>GSHMGGVEVLEVKTGVDAITEVECFLNPEMGDPDENLRGFSLKLSAENDFSSDSPERKMLPCYSTARIPLPNLNEDLTCGNLLMWEAVTVQTEVIGITSMLNLHAGSQKVHEHGGGKPIQGSNFHFFAVGGDPLEMQGVLMNYRTKYPDGTITPKNPTAQSQVMNTDHKAYLDKNNAYPVECWVPDPSRNENTRYFGTFTGGENVPPVLHVTNTATTVLLDEQGVGPLCKADSLYVSAADICGLFTNSSGTQQWRGLARYFKIRLRKRSVKNPYP[5x]

The human polyomavirus BK Virus (BKPyV) is a non-enveloped, double-stranded DNA (dsDNA) virus that belongs to the family Polyomaviridae. A polyomavirus capsid consists of 72 pentamers of the major capsid protein VP1. Gangliosides were found to mediate cell attachment of BKPyV, and gangliosides GD1b and GT1b were later shown to function as specific receptors for BKPyV. Crystal structures of Polyoma, SV40, MCPyV and JCPyV VP1 show that receptors are bound in shallow grooves formed by VP1 loop structures on the outer surface of the virus.

We incubated BKPyV VP1 crystals in 20 mM GD3 oligosaccharide solution and solved the structure of the resulting complex at 1.7 Å resolution. The structures of unliganded and liganded BKPyV VP1 are virtually identical (r.m.s.d. of 0.4 Å for all atoms of one monomer), indicating that GD3 binding does not induce a conformational change in the protein. GD3 engages BKPyV VP1 at the top of the pentamer, which corresponds to the outer surface of the virion. Contacts involve residues in the BC1-, HI- and DE-loops of one monomer, as well as the BC2-loop of the clockwise neighboring VP1 monomer (BC2cw) and the DE-loop of the counterclockwise neighbor (DEccw). In both cases, only the terminal NeuNAc-α2,8-NeuNAc motif interacts with BKPyV VP1, while the Gal-Glc moiety projects into solution. The terminal NeuNAc 4R is the main contact of GD3 with BKPyV VP1. The sialic acid carboxylate group is recognized by two hydrogen bonds to the side chains of S274 and T276. The second sialic acid of GD3, NeuNAc 3R, has weaker electron density and makes fewer contacts with the protein. Its carboxylate group forms a salt bridge with the K68 side chain. BKPyV VP1 specificity for the α2,8-disialyl motif can be attributed to residues K68 and H138, which form contacts with the internal NeuNAc 3R.> PQFHLWKRPVVTAHIEGQPVEVLLDTGADDSIVTGIELGPHYTPKIVGGIGGFINTKEY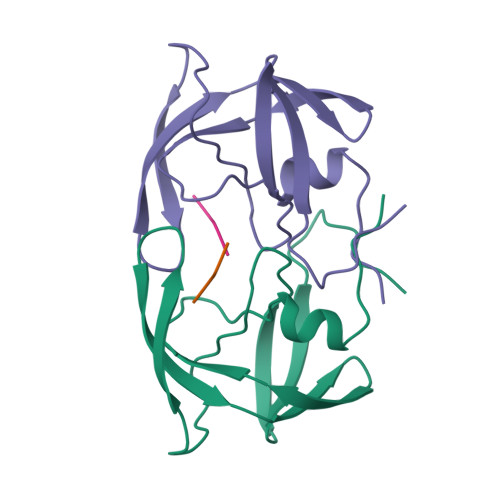KNVEVEVLGKRIKGTIMTGDTPINIFGRNLLTALGMSLNF;> FLEK>[4x]MEVKKFKRFESYKRDNQLPPKVRDMGIVIDQKNNTIVLPIMGRPVPFHINTIKNASKSDEGEWSFLRINFLSPGQGVGRKDDQP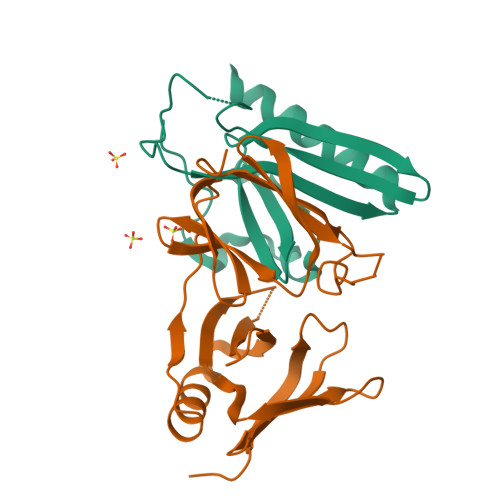FEDASAHFVRSLTFRSTDGDRYAEIANQISNLKREAVKREQEK;>GSHMAAIESFDHIYLDLSKEPGKCRFAENGLGWKPVGGGETFTLDVSNIGGAQWSRAARGYEVKILQRTSGVIQLDGFQQEDYERLAKIFKNWYSTNLENKEHSLRGWNWGKAEFGKAELTFNVQNRPAFEIPYSEIANTNLAGRNEIAVEFAPGDHGKSSQNGQVKSKKASASRDQLVEIRFYIPGTTTRKEAE[4x]>MRLQKDFDRVMGIILMILILAIPSLQICNKSYTEGDPVIINPVPGLPVDFIRGVDASEAPWIIELGGKYYDENGVERDLLDILKENGVNWIRLRVWNDPYDEQGRPYGGGNCDLPRMTDFAAKAKAKGFGVLIDFHYSDWWADPSKQSKPKAWANLSYPELVEAVYNWTYNALKYMAEHNALPDMVQIGNEINNGFLWPDGSAANWTQFVGLLKAAISAVKDVNPNIKIVIHLAGVKADFYINFIDRLINSGVSFDVIAISFYPYWHGTMDDFRNLVRTLVQRYDKKILVAETAYAWTLDDSDGHPNIFGSRDLEVKGGYKASIQGQASFIRDLIAALYEEGKDKALGIFYWGATWIPYPGAGWKTGEGNPWENQALFDFNGRA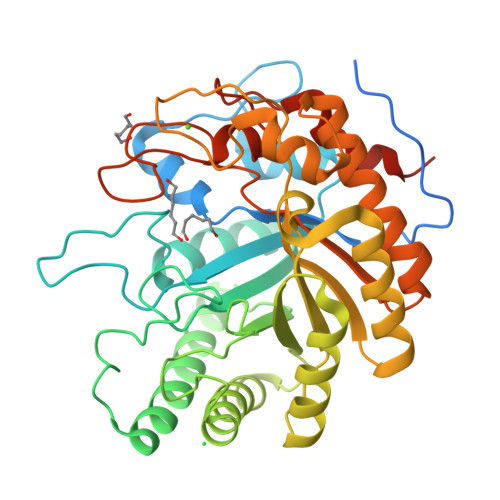LPSLKVFRLVYEAQPVEIKPLEL[2x]The HECT E3 ubiquitin ligases 1 (WWP1) and 2 (WWP2) are responsible for the ubiquitin-mediated degradation of key tumour suppressor proteins and are dysregulated in various cancers and diseases. Two members of the NEDD4 family, WW domain-containing E3 ligase 1 (WWP1) and 2 (WWP2), are of particular interest due to their targeting of the tumour suppressor protein phosphatase and tensin homolog (PTEN) as well as various other tumour suppressors and transcription factors. The HECT-E3 ligases may offer the best druggability as they participate directly in the Ub transfer, unlike the RING-type, and with their catalytic function relying on a single active-site cysteine. We evaluate their structure-activity relationship (SAR) by synthesis aided by molecular docking using X-ray crystal structures of WWP1 and WWP2 solved as part of this study and improved over those previously reported.

However, we were able to solve and refine structures for the apo-proteins which were improvements on previously published data. The available crystal structures for WWP1 (PDB ID: 6J1X20) and WWP2 (PDB ID: 5TJ819) have missing domains and/or high Rfree values. The WWP2-LH crystal structure was solved at a resolution of 2.05 Å in the same space group as that reported in the literature. Unfortunately, however, the WW2 domain was still disordered and therefore missing from the structure. The grid boxes to perform the docking simulations were generated in cavities on the HECT domain surrounding the active site cysteines 890 (WWP1) and 838 (WWP2) given the ability of NSC-217913 to interfere with ubiquitination. The ligand poses of compound 11 in both WWP1-2L34H and WWP2-LH are somewhat similar due to the similarities of the proposed binding site between these two enzymes. These poses show the imidazo[4,5-b]pyrazine moiety engaging in π-π interactions with the phenolic side chain of Tyr639WWP1-2L34H and Tyr587WWP2-LH alongside the Cys640WWP1-2L34H and Cys588WWP2-LH backbone amides participating in hydrogen bonding interactions with the imidazole nitrogen. Against WWP2-LH, the butyrate chain has multiple hydrophobic contacts with the aromatic ring of Tyr587 and the alkyl side chain of Ile813, with the backbone amide from Ile813 also undergoing hydrogen bonding with the carbonyl oxygen of the ester. Lastly, the side chain of Ser646, located at the rear of the cavity, forms a halogen bond with one of the heterocyclic chlorides. Interestingly, all compounds modelled against WWP2-LH also participate in halogen bonding between Ser646 and the same heterocyclic chloride.

> GPGWEKRTDPRGRFYYVDHNTRTTTWQRPTAEYVRNYEQWQSQRNQLQGAMQHFSQRFLYQSSSASQGSPGAYDRSFRWKYHQFRFLCHSNALPSHVKISVSRQTLFEDSFQQIMNMKPYDLRRRLYIIMRGEEGLDYGGIAREWFFLLSHEVLNPMYCLFEYAGKNNYCLQINPASSINPDHLTYFRFIGRFIAMALYHGKFIDTGFTLPFYKRMLNKRPTLKDLESIDPEFYNSIVWIKENNLEECGLELYFIQDMEILGKVTTHELKEGGESIRVTEENKEEYIMLLTDWRFTRGVEEQTKAFLDGFNEVAPLEWLRYFDEKELELMLCGMQEIDMSDWQKSTIYRHYTKNSKQIQWFWQVVKEMDNEKRIRLLQFVTGTCRLPVGGFAELIGSNGPQKFCIDKVGKETWLPRSHTCFNRLDLPPYKSYEQLREKLLYAIEETE>GASMTIEDEYSGPKLEDGKVTISFMKELMQWYKDQKKLHRKCAYQILVQVKEVLSKLSTLVETTLKETEKITVCGDTHGQFYDLLNIFELNGLPSETNPYIFNGDFVDRGSFSVEVILTLFGFKLLYPDHFHLLRGNHETDNMNQIYGFEGEVKAKYTAQMYELFSEVFEWLPLAQCINGKVLIMHGGLFSEDGVTLDDIRKIERNRQPPDSGPMCDLLWSDPQPQNGRSISKRGVSCQFGPDVTKAFLEENNLDYIIRSHEVKAEGYEVAHGGRCVTVFSAPNYCDQM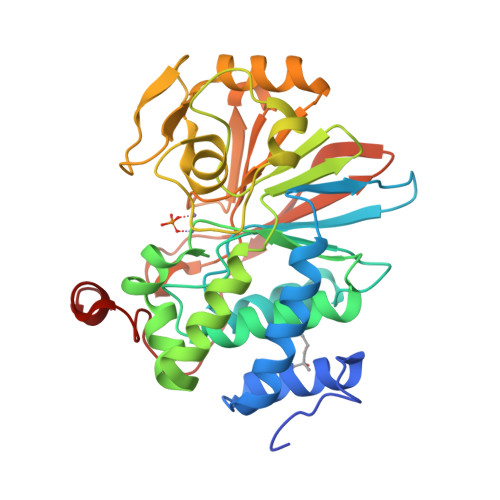GNKASYIHLQGSDLRPQFHQFTAVPHPNVKPMAYANTLLQLGMM[2x]> MTNAALDDKTIVRDYFNSTGFDRWRRIYGDGQVNFVQKDIRVGHQQTVDSVVAWLVADGNLPGLLVCDAGCGVGSLSIPLAQAGALVYGSDIS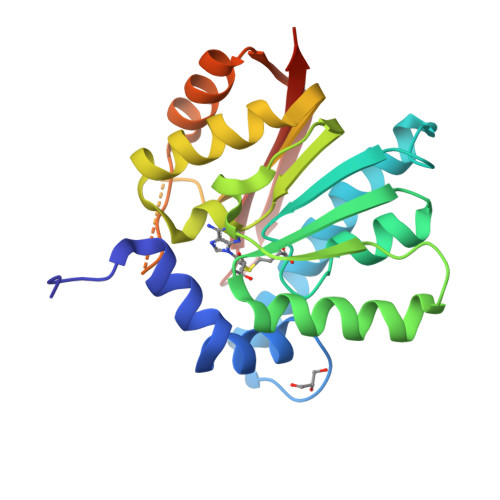EKMVGEAQQKAQEVLAYGNQPTFMTQDLAQLGGKYDTVICLDVLIHYPTEEASAMISHLASLADRRLILSFAPKTLGLTVLKKIGGLFPGPSKTTRAYQHKEADIRKILGDNGFSIARTGMTSTRFYYSRILEAVRSLEHHHHHH> MSQEALKAPVVVLGAGLASVSFVAELRQAGYQGLITVVGDEAERPYDRPPLSKDFMAHGDAEKIRLDCKRAPEVEWLLGVTAQSFDPQAHTVALSDGRTLPYGTLVLATGAAPRALPTLQGATMPVHTLRTLEDARRIQAGLRPQSRLLIVGGGVIGLELAAT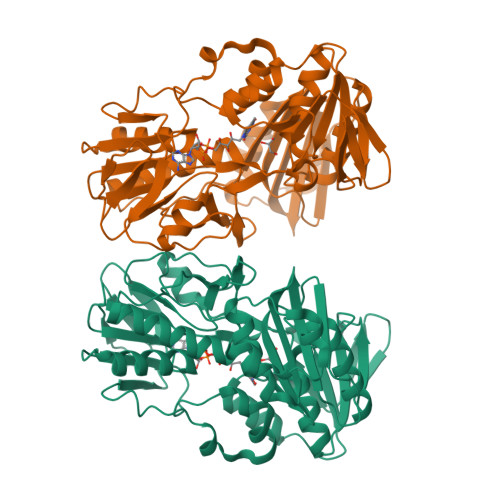ARTAGVHVSLVCTGPRLMSRAAPATLADFVARYHAAQGVDLRFERSVTGSVDGVVLLDDGTRIAADMVVVGIGVLANDALARAAGLACDDGIFVDAYGRTTCPDVYALGDVTRQRNPLSGRFERIETWSNAQNQGIAVARHLVDPTAPGYAELPWYWSDQGALRIQVAGLASGDEEIVRGEVSLDAPKFTLIELQKGRIVGATCVNNARDFAPLRRLLAVGAKPDRAALADPATDLRKLAAAVAA> RAQEDEDGDYEELVLALRSEEDGLAEAPEHGTTATFHRCAKDPWRLPGTYVVVLKEETHLSQSERTARRLQAQAARRGYLTKILHVFHGLLPGFLVKMSGDLLELALKLPHVDY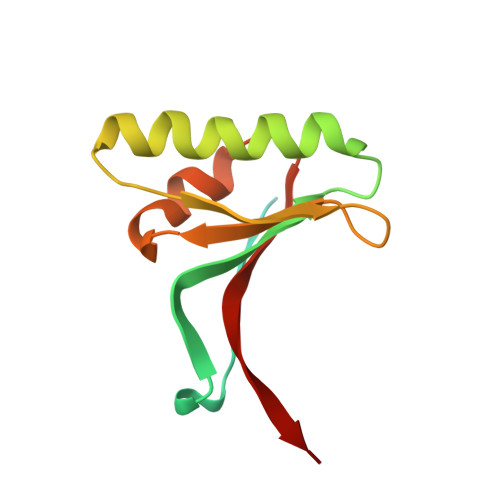IEEDSSVFAQ>MKADAVKIADGVYWVGVLDWDIRMYHGYTLNGTTYNAYLVFGDDKVALIDNTYPGTSAQMWGRIKDACEKEGREFKIDVIVQNHVEKDHSGALPEIHKKFPEAPIYCTEVAVEGLVKHFPSLKGAPFKVVKSLESIDLGGKTLTFLEAPLLHWPDSMFTLYAEEGILFSNDAFGQHLCFTQRFDHEIPENILMDANQKFYANLITPLSKLVLKKFKEVIELGLLEKIKMIAPSHGQIWTDPMKVIGAYQDFATGKCKDKVTIVYDTMHGSTQKMAHAFAEGIMSEGVDVKMYF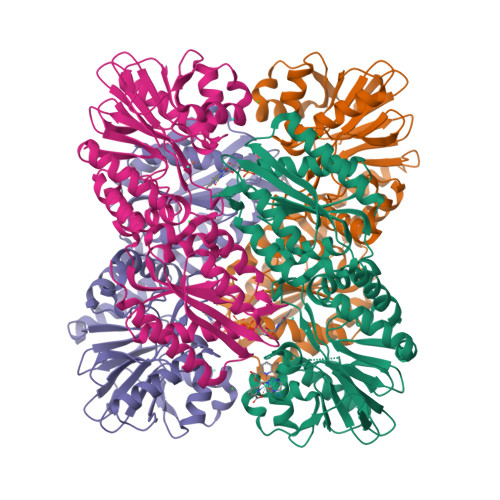LHNDERSEIVKDILDSKAFLLGAPTIYDEPFPSVGDLIYYLKGLKFNRTGLKRLALAFGSMGGNGGGTKVLAEKLKECGFEVLDEYELYYVPTEDELEKCYNMGKRLAVKVKEMKTE[8x]> CDNDTEPGGTAVEKMAGDWWVTVNAFIDGKEVEDPFGAGHLQM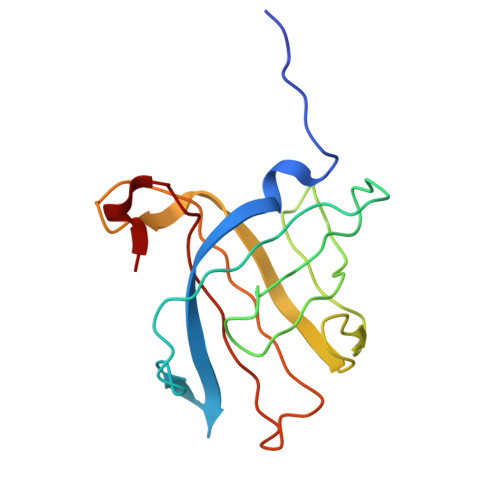STYNTASNSETEMWLDDLGNFWEYKLKVNVNYAARTFSTTGFVDNVTYESKVKITDGKVLEKAATTPSGMPADSIVYMVQFDDDEDGLTYKVSGFRRTGFPADDF>[2x]GAMSQIKLTPEELRSSAQKYTAGSQQVTEVLNLLTQEQAVIDENW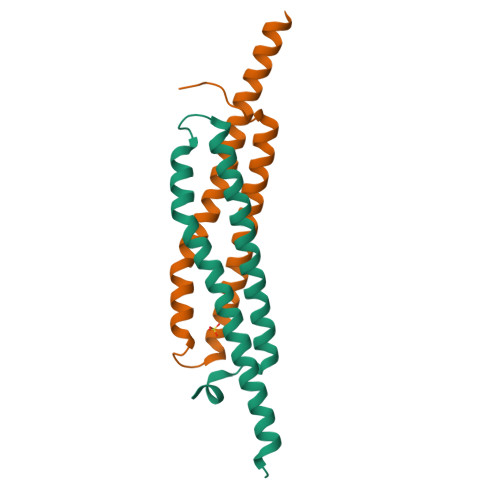DGSTFDSFEAQFNELSPKITEFAQLLEDINQQLLKVADIIEQTDADIASQISG>[2x]MRVAVVGATGAVGREILKVLEARNFPLSELRLYASPRSAGVRLAFRGEEIPVEPLPEGPLPVDLVLASAGGGISRAKALVWAEGGALVVDNSSAWRYEPWVPLVVPEVNREKIFQHRGIIANPNCTTAILAMALWPLHRAFQAKRVIVATYQAASGAGAKAMEELLTETHRFLHGEAPKAEAFAHPLPFNVIPHIDAFQENGYTREEMKVVWETHKIFGDDTIRI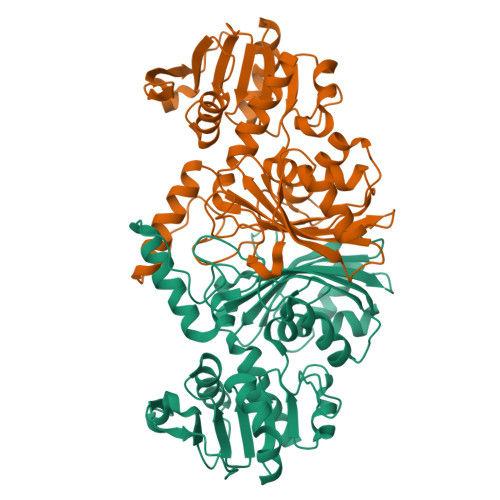SATAVRVPTLRAHAEAVSVEFARPVTPEAAREVLKEAPGVEVVDEPEAKRYPMPLTASGKWDVEVGRIRKSLAFENGLDFFVVGDQLLKGAALNAVQIAEEWLKGA>[4x]AESLPDLKIEKLDEGVYVHTSFEEVNGWGVVPKHGLVVLVNAEAYLIDTPFTAKDTEKLVTWFVERGYKIKGSISSHFHSASTGGIEWLNSRSIPTYASELTNELLKKDGKVQA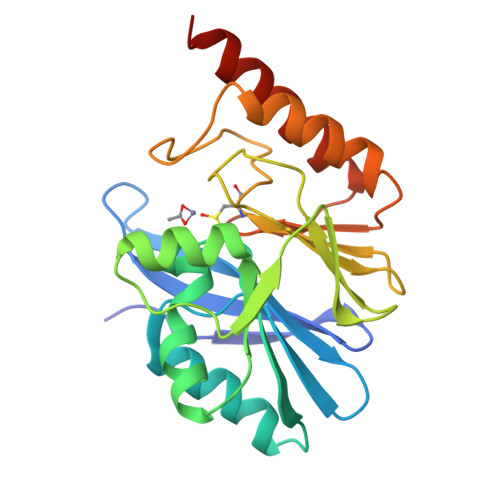TNSFSGVNYWLVKNKIEVFYPGPGHTPDNVVVWLPERKILFGGCFIKPYGLGNLGDANIEAWPKSAKLLKSKYGKAKLVVPSHSEVGDASLLKLTLEQAVKGLNESKKPSKPSN>MGSSHHHHHHSQDPKPRVLVLTGAGISAESGIRTFRAADGLWEEHRVEDVGTPEGFDRDPELVQAFYNARRRQLQQPEIQPNAAHLALAKLQDALGDRFLLVTQNCDNLHERAGNTNVIHMHGELLKVRCSQSGQALDWTGDVTPEDKCHCCQFPAPLRPHVVWFGEMPLGMDEIYMALSMADIFIAIGTSGHVYPAAGFVHEAKLHGAHTVELNLEPSQVGNEFAEKY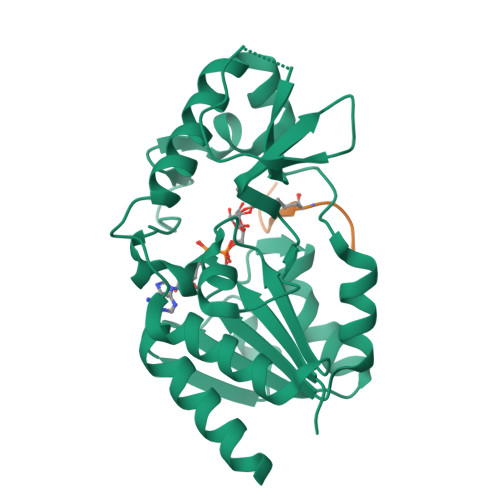YGPASQVVPEFVEKLLKGLKAGSIA[4x];>[4x]KGGAKRHRKIL> SNAMLFCDDSKKYLKEQNINLKNEFDKDDKRVEKFSLKHQNIYFDYSKNLINDYILKSLLESAEKSSLKDKIKQMFNGAKINSTEHRAVLHTALRDLSSTPLIVDGQDIRQEVTKEKQRVKELVEKVVSGRWRGFSGKKITDIVNIGIGGSDLGPKMVVRALQPYHCTDLKVHFVSNVDADSLLQALHVVDPETTLLIIASKSFSTEETLLNSISAR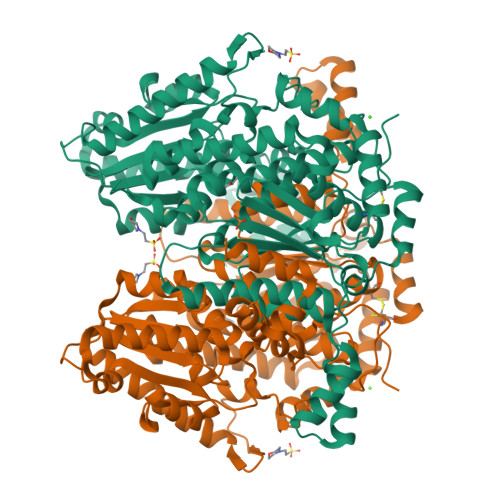EWLLDHYEDEKAVANHFVAISSKLDKVKEFGIDLEHCYKMWDWVGGRYSLWSSIGMSIAFAIGYDNFEKLLAGAYSVDKHFKETEFSKNIPVIMALLASYYSCTYNSQSQALLPYDERLCYFVDYLQQADMESNGKSVNIAGETVNYQTGVVLWGGVGTNGQHAFHQLLHQGNIFIPVDFIAIATSHHNYDNHQQALLANCFAQSQALMFGQSYDMVYNELLKSGLNETQAKELAAHKVIPGNRPSTTILLDELSPYSLGALIALYEHKIFVQGVLWDINSYDQWGVELGKKLGKNILKAMNDDSSDEYQNLDDSTRQLIAKVKNK>MTKTFKTLDDFLGTHFIYTYDNGWEYEWYAKNDHTVDYRIHGGMVAGRWVTDQKADIVMLTEGIYKISWTSPTGTDVALDFMPNEKKLHGTIFFPKWVEEHPEITVTYQNEHIDLMEQSREKYATYPKLVVPEFANITYMGDAGQNNEDVISEAPYKEMPNDIRN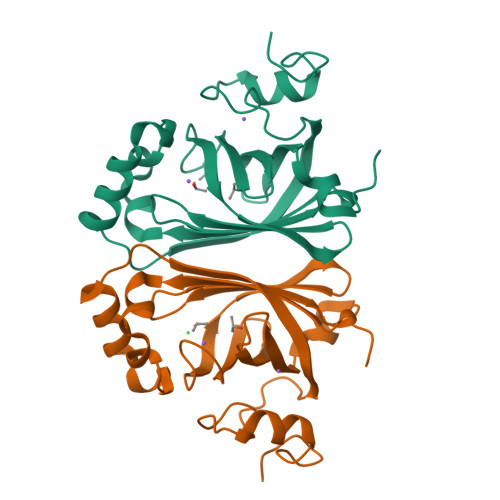GKYFDQNYHRLNK[2x]>[2x]MPGEEVSQAKQQLKLIIDPYLSVSEVEKVLAACDFGDLAHTGITRKSGEPYILHPIAVSCILANMRLDPETLMAALLHDVIEDTQYTKDDIIERFGQTVAELVDGVTKLSQSSDKEYNKAASFRKILQATLQDPRVIIIKLADRYHNMTTLGALRPDKRARIAQETFDIFVPMA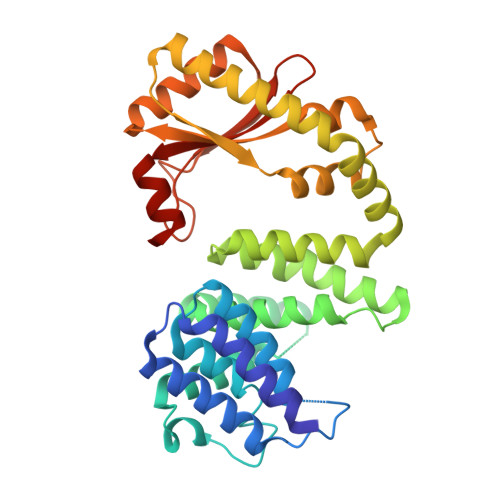RLVGMNEMADNLENLCYQNLDLDMFDNVQNALLQTKPERCKYQSIWEQNLAELLHNYHIQGRIKKKNNNIELLRHFVKNEMDLQELTHSHAFEIVLQSIADCDRLVAALKENFQVIQYQDHIRRPLPGGNQSLMIKLKGEKTTLSLTIQTELMRKAARFGVVLG> AMADIGSEFGHRTLASTPALWASIPCPRSELRLDLVLPSGQSFRWREQSPAHWSGVLADQVWTLTQTEEQLHCTVYRGDKSQA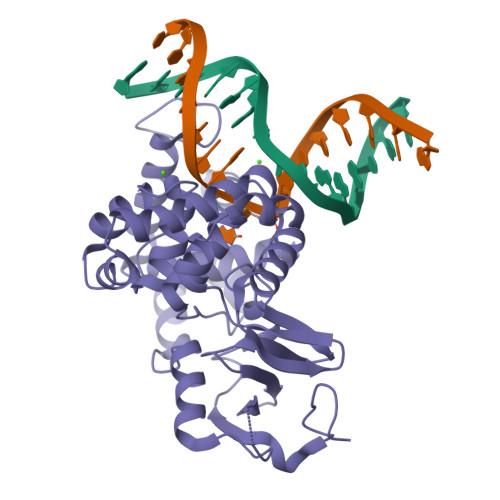SRPTPDELEAVRKYFQLDVTLAQLYHHWGSVDSHFQEVAQKFQGVRLLRQDPIECLFSFICSSNNNIARITGMVERLCQAFGPRLIQLDDVTYHGFPSLQALAGPEVEAHLRKLGLGYRARYVSASARAILEEQGGLAWLQQLRESSYEEAHKALCILPGVGTQVADCICLMALDKPQAVPVDVHMWHIAQRDYSWHPTTSQAKGPCPQTNKELGNFFRSLWGPYAGWAQAVLFSADLRQSR>MLWKKSLSELRELLKRGEVSPKEVVESFYDRYNQTEEKVKAYITPLYGKALKQAESLKERELPLFGIPIAVKDNILVEGEKTTCASKILENFVAPYDATVIERLKKAGALIVGKTNLDEFAMGSSTEYSAFFPTKNPWDLERVPGGSSGGSAASVAVLSAPVSLGSDTGGSIRQPASFCGVIGIKPTYGRVSRYGLVAFASSLDQIGVFGRRTEDVALVLEVISGWDEKDSTSAKVPVPEWSEEVKKEVKGLKIGLPKEFFEYELQPQVKEAFENFIKELEKEGFEIKEVSLPHVKYSIPTYYIIAPSEASSNLARYDGVRYGYRAKEYKDIFEMYARTRDEGFGPEVKRRIMLGTFALSAGYYDAYYLKAQKVRRLITNDFLKAFEEVDVIASPTTPTLPFKFGERLENPIEMYLSDILTVPANLAGLPAISIPIAWKDGLPVGGQLIGKHWDETTLLQISYLWEQKFKHYEKIPLT[8x];>[8x]MNEKYEAVIGLEIHVQMDTKTKMFCGCKVEFGAEPNTNVCPVCLGMPGALPIVNKRAVEYAIRASLALNCEVHEESVFARKHYFYPDLPKGYQISQYEKPLATNGWVELNLPNGEKKKVRIRRLHIEEDAGKNIHEGDKTLVDLNRAGTPLMEIVTEPDIRTPEEARLFLEKLRNIMRYAGVSKADMEKGQLRCDINVSIRPKGSKEFGTRVEIKNVNSFRFVQKALEYEIERQINVVEEGGEVVQETRTFDPQTGKTYPMRTKEEAEDYRYFPDPDLVPLKVKKEWIEEIKKNMPELPDQRFERLIKEYGLSEYEAGILVNHKEVGDFFEEAVRHFKEPKGIVNWLINDLLGLLRDKGISIEESPVKPEHLAELVKLIKEKVISTKIGKEVIKEMVETGKTPSQIVEEKGLKQITDENQIKELVKKIFEKHPKEV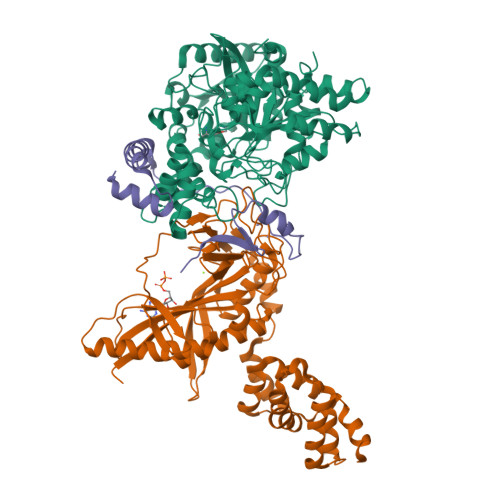ERLKQGEEKLIGFFVGQVMRETRGKANPQVVNKVIRELVKEV;>MVDREWVLKIAKLARLELKEEEIEVFQKQLSDILDFIDQLKELDTENVEPYIQEFEETPMREDEPHPSLDREKALMNAPERKDGFFVVPRVVEV[8x]>ANKPMQPITSTANKIVWSDPTRLSTTFSASLLRQRVKVGIAELNNVSGQYVSVYKRPAPKPEGCADACVIMPNENQSIRTVISGSAENLATLKAEWETHKRNVDTLFASGNAGLGFLDPTAAIVSSDT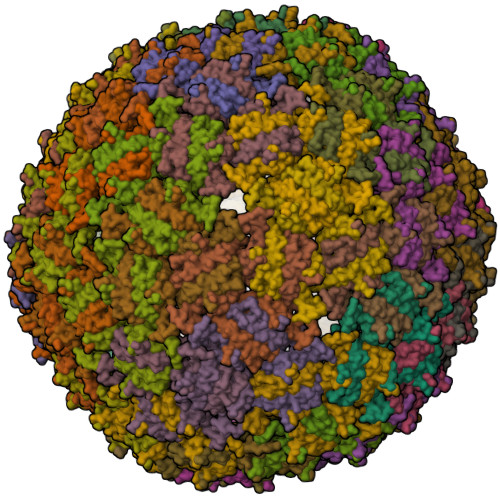T[180x]>[2x]ITGQAACPESWIGFQRK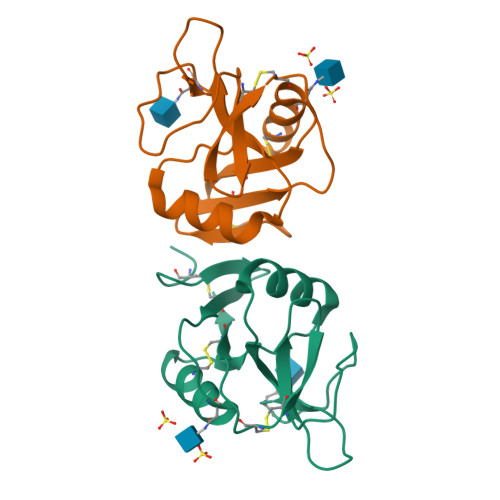CFYFSDDTKNWTSSQRFCDSQDADLAQVESFQELNFLLRYKGPSDHWIGLSREQGQPWKWINGTEWTRQFPILGAGECAYLNDKGASSARCYTERKWICSKSDIHVGTKHHHHHHHHG;>[4x]ETGGLLNCPIYWQQLREKCLLFSHTVNPWNNSLADCSTKESSLLLIRDKDELIHTQNLIRDKAILFWIGLNFSLSEKNWKWINGSFLNSNDLEIRGDAKENSCISISQTSVYSEYCSTEIRWICQKELTPVRNKVYPDSKHHHHHH> MQAQDWAGIPVPADPGNGKQWKLQADMSDDFNYDFPANKEETYIAGKWKNFWHNSWDGPGPTQWRHENVSVSNGHMNIVASRNGNTKTFRNSHDGTYHTLPATQMGCVVSKGHVQYPVFVEARVKIADAVFANNVWMISDDDYEEIDI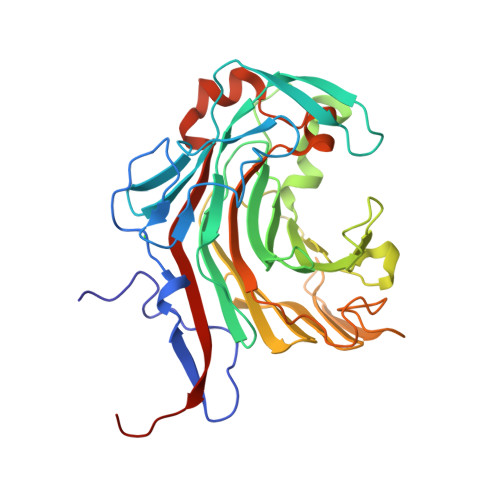CENYGGLGDPGRTGTAMNAWFAKHIHLSHHVFNNRHLTNFDDYQPRDEEGVYGTWYYENGRTDWAGEYSTIGVYWKDPNHLEYYINGKWVRTLSGKNYSYLDPDGKLIEASADFNVLDKYNYTNGKGLTKPMKLIINIEAQDWNALAGRYPTDGEIYGRPEDHIMKVDWIRVYTPEVVTGHHHHHH>MLPSTIQTLTLFLTSGGVLLSLYVSASLSYLLYSDILLKFSPTEITAPTMPLDCANASNVQAVNRSATKGVTLLLPEPEWTYPRLSCPGSTFQKALLISPHRFGETKGNSAPLIIREPFIACGPNECKHFALTHYAAQPGGYYNGTRGDRNKLRHLISVKLGKIPTVENSIFHMAAWSGSACHDGKEWTYIGVDGPDNNALLKVKYGEAYTDTYHSYANKILRTQESACNCIGGNCYLMITDGSASGVSECRFLKIREGRIIKEIFPTGRVKHTEECTCGFASNKTIECACRDNSYTAKRPFVKLNVETDTAEIRLMCTDTYLDTPRPNDGSITGPCESNGDKGSGGIKGGFVHQRMESKIGRWYSRTMSKTERMGMGLYVKYDGDPWADSDALAFSGVMVSMKEPGWYSFGFEIKDKKCDVPCIGIEMVHDGGKETWHSAATAIYCLMGSGQLLWDTVTGVDMAL[2x]

The neuraminidase inhibitors (NAIs) oseltamivir and zanamivir are the antiviral agents available in France to treat influenza A or B virus infections. The NA active site includes catalytic residues (R118, D151, R152, R224, E276, R292, R371, and Y406; N2 numbering) that interact directly with the sialic acid substrate and framework residues (E119, R156, W178, S179, D/N198, I222, E227, H274, E277, N294, and E425; N2 numbering) that stabilize the active site. NAs are divided into 3 phylogenic groups: influenza B viruses, group 1 (N1, N4, N5, and N8), and group 2 (N2, N3, N6, N7, and N9) from influenza A viruses. I221 (B NA numbering), I222 (N2 numbering), and I223 (N1 numbering) amino acids are highly conserved framework residues in NAs of influenza viruses.

We used X-ray crystallography to understand the structural basis of resistance to oseltamivir conferred by NA carrying the I221L substitution.>[2x]GPKFPRVKNWELGSITYDTLCAQSQQDGPCTPRRCLGSLVLPRKLQTRPSPGPPPAEQLLSQARDFINQYYSSIKRSGSQAHEERLQEVEAEVASTGTYHLRESELVFGAKQAWRNAPRCVGRIQWGKLQVFDARDCSS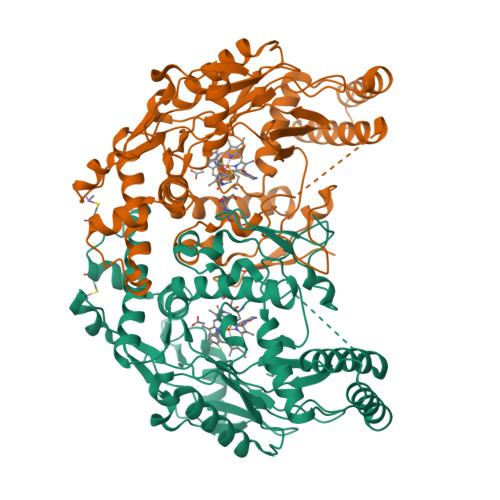AQEMFTYICNHIKYATNRGNLRSAITVFPQRAPGRGDFRIWNSQLVRYAGYRQQDGSVRGDPANVEITELCIQHGWTPGNGRFDVLPLLLQAPDEAPELFVLPPELVLEVPLEHPTLEWFAALGLRWYALPAVSNMLLEIGGLEFSAAPFSGWYMSTEIGTRNLCDPHRYNILEDVAVCMDLDTRTTSSLWKDKAAVEINLAVLHSFQLAKVTIVDHHAATVSFMKHLDNEQKARGGCPADWAWIVPPISGSLTPVFHQEMVNYILSPAFRYQPDPW Kinesin-1 transports numerous cellular cargoes along microtubules. The kinesin-1 light chain (KLC) mediates cargo binding and regulates kinesin-1 motility. KLC comprises an N-terminal heptad repeat region that oligomerizes with the KHC stalk, an acidic linker region, and a tetratricopeptide repeat (TPR) domain containing six TPRs (TPR1-6) (Gauger and Goldstein, 1993, Verhey et al., 1998, Wong and Rice, 2010, Zhu et al., 2012). The KLC TPR domain (KLCTPR) is unusual in binding to multiple ligands using distinct sites (Hammond et al., 2008, Zhu et al., 2012).

Certain cargo molecules bind to the KLCTPR using tryptophan-acidic motifs, which bind to the inner concave surface of the KLCTPR, spanning TPRs 2–4 (Araki et al., 2007, Dodding et al., 2011, Kawano et al., 2012, Pernigo et al., 2013, Zhu et al., 2012). Tryptophan-acidic cargoes activate kinesin-1 by releasing the KLC LFP motif from the KLCTPR (Yip et al., 2016). Intriguingly, TPR1 forms a similar dimer interface in all crystal structures of the full-length KLCTPR (Nguyen et al., 2017). Notably, we also found the same interface in our previously unpublished, 4-Å crystal structure of the KLC2TPR bound to a tryptophan-acidic peptide derived from calsyntenin-1 (CSTN-WD2) (Araki et al., 2007). The TPR1:TPR1 packing interaction is unique in being found in every copy of the KLC1TPR and KLC2TPR in all crystal structures, suggesting that it is independent of crystallographic environment or crystallization conditions. The amino acid residues that form the crystallographic TPR1:TPR1 interfaces are totally conserved in essentially all Bilateria and over half of the non-Bilaterian species in our datasets, across all phyla. These observations suggest that the TPR1:TPR1 interfaces observed in crystals of the KLCTPR are not simply crystal packing artifacts and may be functionally relevant. Thus, the KLCTPR possesses the propensity to self-associate via TPR1 in a manner that mimics JIP3LZ domain binding.

>[2x]GRGYEIPARLRTLHNLVIQYASQGRYEVAVPLCKQALEDLEKTSGHDHPDVATMLNILALVYRDQNKYKDAAHLLNDALAIREKTLGKDHPAVAATLNNLAVLYGKRGKYKEAEPLCKRALEIREKVLGKFHPDVAKQLSNLALLCQNQGKAEEVEYYYRRALEIYATRLGPDDPNVAKTKNNLASCYLKQGKYQDAETLYKEILTRAHEKEFGSVNGENKPIWMHAEEREESKDKRRDSAPYGEYGSWYKACKVDSPTVNTTLRSLGALYRRQGKLEAAHTLEDCASRSRKR;>NATRQLEWDDSTLSY[2x]>MSNLSKGTGSRKDTKMRIRAFPMTMDEKYVNSIWDLLKNAIQEIQRKNNSGLSFEELYRNAYTMVLHKHGEKLYTGLREVVTEHLINKVREDVLNSLNNNFLQTLNQAWNDHQTAMVMIRDILMYMDRVYVQQNNVENVYNLGLIIFRDQVVRYGCIRDHLRQTLLDMIARERKGEVVDRGAIRNACQMLMILGLEGRSVYEEDFEAPFLEMSAEFFQMESQKFLAENSASVYIKKVEARINEEIERVMHCLDKSTEEPIVKVVERELISKHMKTIVEMENSGLVHMLKNGKTEDLGCMYKLFSRVPNGLKTMCECMSSYLREQGKALVSEEGEGKNPVDYIQGLLDLKSRFDRFLLESFNNDRLFKQTIAGDFEYFLNLN[5x];>MAENHCELLSPARGGIGAGLGGGLCRRCSAGLGALAQRPGSVSKWVRLNVGGTYFLTTRQTLCRDPKSFLYRLCQADPDLDSDKDETGAYLIDRDPTYFGPVLNYLRHGKLVINKDLAEEGVLEEAEFYNITSLIKLVKDKIRERDSKTSQVPVKHVYRVLQCQEEELTQMVSTMSDGWKFEQLVSIGSSYNYGNEDQAEFLCVVSKELHNTPYGTASEPSEKAKILQERGSRM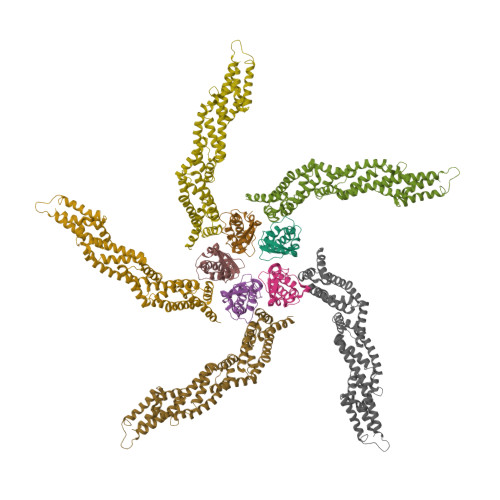[5x]>GAMDPEFGRPMEISDKISKEEMVRRLKMVVKTFMDMDQDSEEEKELYLNLALHLASDFFLKHPDKDVRLLVACCLADIFRIYAPEAPHTSPDKLKDIFMFITRQLKGLEDTKSPQFNRYFYLLENIAWVKSYNICFELEDSNEIFTQLYRTLFSVINNGHNQKVHMHMVDLMSSIICEGDTVSQELLDTVLVNLVPAHKNLNKQAYDLAKALLKRTAQAIEPYITNFFNQVLMLGKTSISDLSEHVFDLILELYNIDSHLLLSVLPQLEFKLKSNDNEERLQVVKLLAKMFGAKDSELASQNKPLWQCYLGRFNDIHVPIRLECVKFASHCLMNHPDLAKDLTEYLKVRSHDPEEAIRHDVIVSIVTAAKKDILLVNDHLLNFVRERTLDKRWRVRKEAMMGLAQIYKKYALQSAAGKDAAKQIAWIKDKLLHIYYQNSIDDRLLVERIFAQYMVPHNLETTERMKCLYYLYATLDLNAVKALNEMWKCQNLLRHQVKDLLDLIKQPKTDASVKAIFSKVM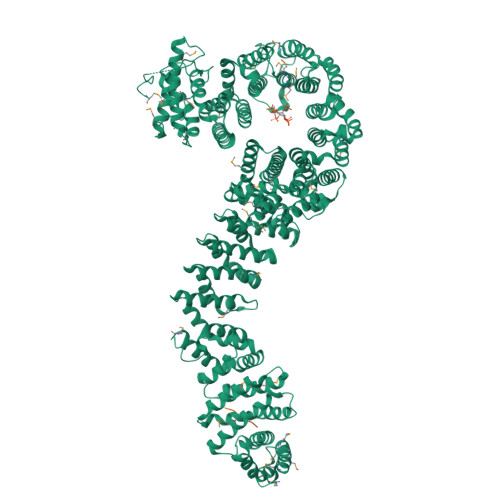VITRNLPDPGKAQDFMKKFTQVLEDDEKIRKQLEVLVSPTCSCKQAEGCVREITKKLGNPKQPTNPFLEMIKFLLERIAPVHIDTESISALIKQVNKSIDGTADDEDEGVPTDQAIRAGLELLKVLSFTHPISFHSAETFESLLACLKMDDEKVAEAALQIFKNTGSKIEEDFPHIRSALLPVLHHKSKKGPPRQAKYAIHCIHAIFSSKETQFAQIFEPLHKSLDPSNLEHLITPLVTIGHIALLAPDQFAAPLKSLVATFIVKDLLMNDRLPGKKTTKLWVPDEEVSPETMVKIQAIKMMVRWLLGMKNNHSKSGTSTLRLLTTILHSDGDLTEQGKISKPDMSRLRLAAGSAIVKLAQEPCYHEIITLEQYQLCALAINDECYQVRQVFAQKLHKGLSRLRLPLEYMAICALCAKDPVKERRAHARQCLVKNINVRREYLKQHAAVSEKLLSLLPEYVVPYTIHLLAHDPDYVKVQDIEQLKDVKECLWFVLEILMAKNENNSHAFIRKMVENIKQTKDAQGPDDAKMNEKLYTVCDVAMNIIMSKSTTYSLESPKDPVLPARFFTQPDKNFSNTKNYLPPEMKSFF[2x];> MTSRFGKTYSRKGGNGSSKFDEVFSNKRTTLST3-[(E)-2-(2-chloro-4-{[3-{[(R)-(2,6-dichlorophenyl)(hydroxy)-lambda~4~-sulfanyl]methyl}-5-(1-methylethyl)isoxazol-4-yl]methoxy}phenyl)ethenyl]benzoic 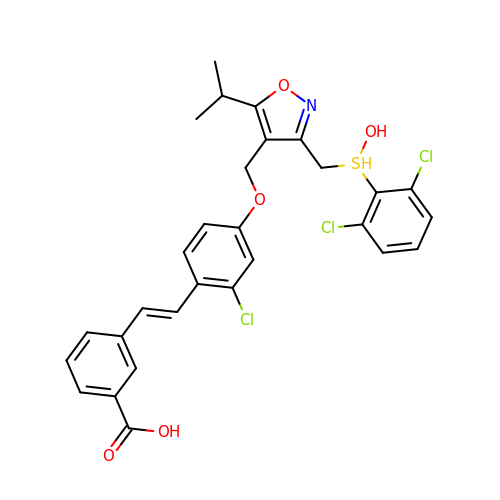acid | C29 H26 Cl3 N O5 S | MUAOISKUROHRCK-MDZDMXLPSA-N> GMSAKDVFHQVVKIALEKDGWQITNDPLTISVGGVNLSIDLGAEKLIAAEREGEKIAVEVKSFLERS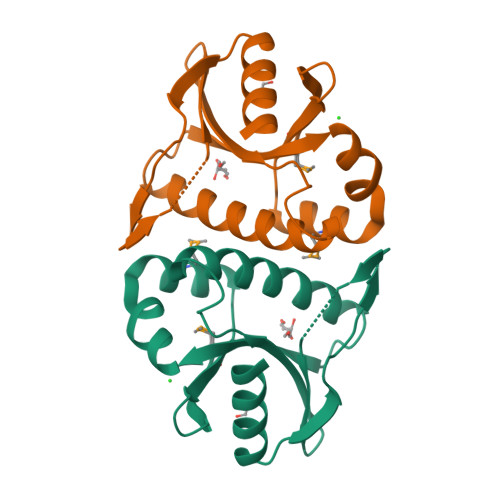SAISEFHTALGQFINYRGALRRRQPERVLYLAVPLTTYKTFFQLDFPKEMIAENQVKMLIYDVEQEVIFQWIN Haloarchaeal pleomorphic viruses (HRPVs) infect archaeal hosts living in hypersaline environments. The virions contain two major protein species, a spike protein (VP4 and VP4-like proteins) protruding from the membrane surface and a smaller membrane associated protein (VP3 and VP3-like proteins) residing mostly inside the virion. Here we describe crystallographic structures of VP4-like spike proteins from two pleolipoviruses, HRPV-2 and HRPV-6, showing that these proteins have a unique fold, different from class I–III fusion proteins. VP5 is thus a bona fide fusion protein.

To determine the low-resolution structure and oligomeric state of VP5 on the HRPV-6 surface, we used cryo-electron tomography and sub-tomogram averaging. This was facilitated by Volta phase plate technology, which provided sufficient contrast in the tomographic reconstructions for identification and alignment of the relatively small VP5 (~57 kDa) spikes. Sub-tomogram averaging of 8953 manually picked spikes resolved the VP5 structure in situ at 16-Å resolution, as estimated by Fourier shell correlation (0.143 threshold). Each virion (N = 247) had 35 ± 7 VP5 spikes on the surface and each spike is a monomer with the characteristic triangular shape reminiscent of that seen in the high-resolution X-ray structures. We fitted the VP5 X-ray structure into the 16-Å resolution VP5 tomographic density as a rigid body. Although the fitting is generally robust (cross-correlation coefficient 0.84), there is additional density in the groove between the N- and C-terminal domains, which slightly protrudes from the EM density, suggesting that VP5 attached to the viral membrane may adopt a more compact conformation than in the crystal. The C-terminus is proximal to the viral membrane, consistent with the predicted C-terminal transmembrane region anchoring VP5 to the membrane. Density corresponding to the last 39 residues of HRPV-6 VP5 is not observed: the 23 residues preceding the very last two C-terminal asparagine residues correspond to the TM domain, and the preceding 19 missing residues (glycine rich) would act to link the ectodomain to the TM domain. In this model, rigid body fitting placed Val461 close to the membrane but this assertion remains to be validated experimentally. The variable, putative receptor binding N2 subdomain is located at the top of the spike.

> IAPLVGYAIGAAAISAVGGIGVGWTLREFEVVGSDDPAEGLTPDVLRNQLSDSVVKRKSNNQSTMVDNQNILDGVEHTAYTEAKIAAIEELNAGSSESAVLSAANSAIDSYETTVRTNFYKSWNETVRELEAMTQTVIAHADVGLSYITDFGDPRFGNLASGTSPNTLKDTTVSMPDGTNFTLLTFRHNTGWDSGNAAYSVVEYNPKEVVTSTNSNTYNTVDGTQYMKFSEWNAVETEMDTVFQNVRNGISTWVTNVYGDVQSGAIEISDLVTPRERATMMAQEEGMSQAIADLIALNVPVDAEREATITIQDTGATLPGTFALTDSSDGPLSAGQTYDPSTFSGDVYFTADMSLVEGPWDAINSGVDGGTITITSEPYEGTAIEVTTVESETVSVPAADWTDNGDGTWSYDASGDLETTITNVDSARFVSTATETTYDTLQLKGAFTVDKLVNKQSGEEVSSTSFTSSEPQTDSNYITQDEWDQLEQQNKELIEKYEQSQSGGGLDLGGLDMFGVPGEMVAVGAAAVIGFLMLGNN> QSACTLQSETHPPLTWQKCSSGGTCTQQTGSVVIDANWRWTHATNSSTNCYDGNTWSSTLCPDNETCAKNCCLDGAAYASTYGVTTSGNSLSIGFVTQSAQKNVGARLYLMASDTTYQEFTLLGNEFSFDVDVSQLPCGLNGALYFVSMDADGGVSKYPTNTAGAKYGTGYCDSQCPRDLKFINGQANVEGWEPSSNNANTGIGGHGSCCSEMDIWEANSISEALTPHPCTTVGQEICEGDGCGGTYSDNRYGGTCDPDGCDWNPYRLGNTSFYGPGSSFTLDTTKKLTVVTQFETSGAINRYYVQNGVTFQQPNAELGSYSGNELNDDYCTAEEAEFGGS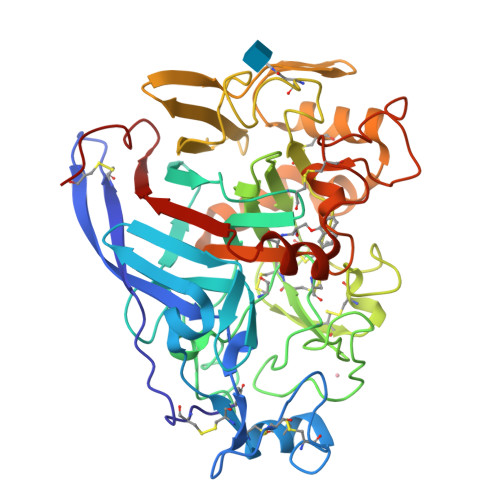SFSDKGGLTQFKKATSGGMVLVMSLWDDYYANMLWLDSTYPTNETSSTPGAVRGSCSTSSGVPAQVESQSPNAKVTFSNIKFGPIGSTGNPSG> VPRGSAKGDGVTDDTAALTSALNDTPVGQKINGNGKTYKVTSLPDISRFINTRFVYERIPGQPLYYASEEFVQGELFKITDTPYYNAWPQDKAFVYENVIYAPYMGSDRHGVSRLHVSWVKSGDDGQTWSTPEWLTDLHPDYPTVNYHCMSMGVCRNRLFAMIETRTLAKNALTNCALWDRPMSRSLHLTGGITKAANQRYATIHVPDHGLFVGDFVNFSNSAVTGVSGDMTVATVIDKDNFTVLTPNQQTSDLNNAGKNWHMGTSFHKSPWRKTDLGLIPSVTE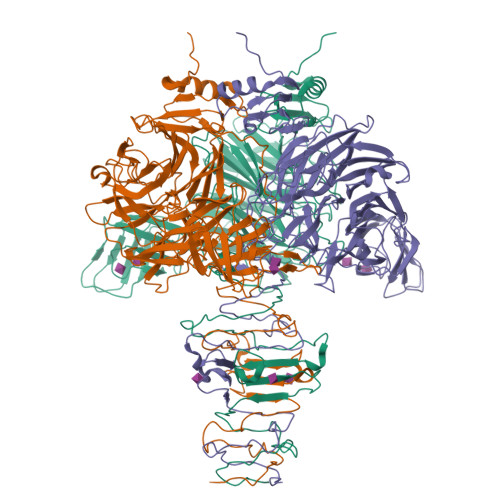VHSFATIDNNGFAMGYHQGDVAPREVGLFYFPDAFNSPSNYVRRQIPSEYEPDASEPCIKYYDGVLYLITRGTRGDRLGSSLHRSRDIGQTWESLRFPHNVHHTTLPFAKVGDDLIMFGSERAENEWEAGAPDDRYKASYPRTFYARLNVNNWNADDIEWVNITDQIYQGGIVNSGVGVGSVVVKDNYIYYMFGGEDHFNPWTYGDNSAKDPFKSDGHPSDLYCYKMKIGPDNRVSRDFRYGAVPNRAVPVFFDTNGVRTVPAPMEFTGDLGLGHVTIRASTSSNIRSEVLMEGEYGFIGKSIPTDNPAGQRIIFCGGEGTSSTTGAQITLYGANNTDSRRIVYNGDEHLFQSADVKPYNDNVTALGGPSNRFTTAYLGSNPIVT3-(4-bromophenyl)propanoic acid | C9 H9 Br O2 | 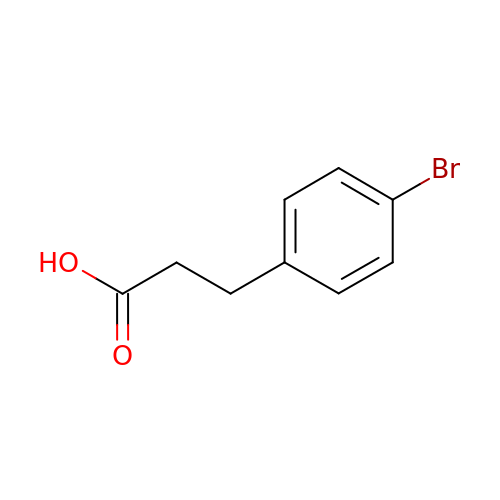NCSTWHYWOVZDOC-UHFFFAOYSA-N>MASGSNVEEYELDVEALVVILRDRNIPRNPLHGEVIGLRLTEGWWGQIERFQMVRLILQNDDNEPLQRPRYEVIQRAVNPHTMFMISGPLAELQLAFQDLDLPEGPLRFGPLANGHYVQGDPYSSSYRPVTMAETAQMTRDELEDVLNTQSEIEIQMINLLELYEVETRALRRQLAERSSTGQGGISPGAPRSRPPVSSFSGLPSLPSIPGIHPRAPSPPRATSTPGNIPWSLGDDNPPSSSFPGPSQPRVSFHPGNPFVEEEGHRPRSQSRERRREILPAPVPSAPPMIQYIPVPPPPPIGTVIPIQHIRSVTGEPPRNPREIPIWLGRNAPAIDGVFPVTTPDLRCRIINAILGGNIGLSLTPGDCLTWDSAVATLFIRTHGTFPMHQLGNVIKGIVDQEGVATAYTLGMMLSGQNYQLVSGIIRGYLPGQAVVTALQQRLDQEIDDQTRAETFIQHLNAVYEILGLNARGQSIRASVTPQPRPSRGRGRGQNTSRPSQGPANSGRGRQRPASGQSNRGSSTQNQNQDNLNQGGYNLRPRTYQPQRYGGGRGRRWNDNTNNQESRPSDQG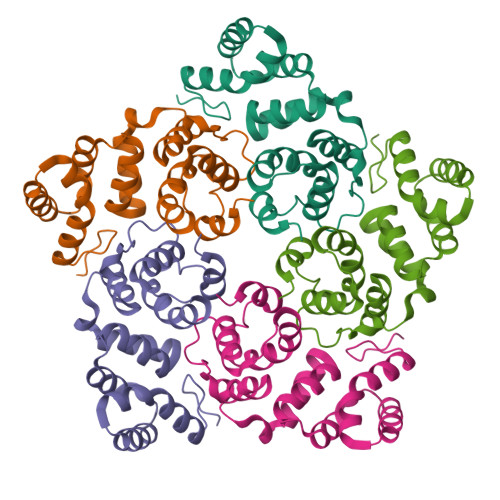SQTPRPNQAGSGVRGNQSQTPRPAAGRGGRGNHNRNQRSSGAGDSRAVNTVTQSATSSTDESSSAVTAASGGDQRD[5x]>[4x]SAKDPVSARMDNDTAALLERIRSDWAR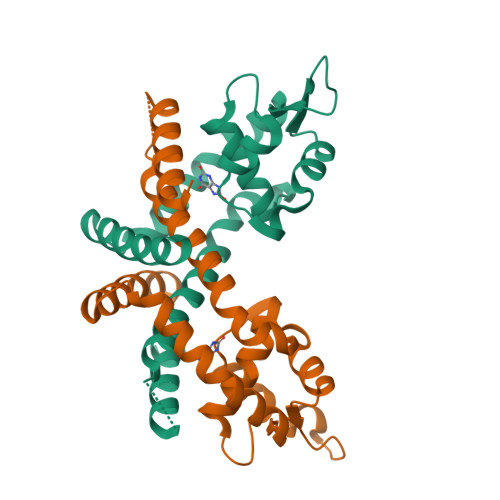LNHGQGPDSDGLTPSAGPMLTLLLLERLHAALGREIERTYAASGLNAAGWDLLLTLYRSAPPEGLRPTELSALAAISGPSTSNRIVRLLEKGLIERREDERDRRSASIRLTPQGRALVTHLLPAHLATTQRVLAPLSAQEQRTLEELAGRMLAGLEQGV> TRYIPDEADFLLGMATVNNCVSYRNPAEGTWYIQSLCQSLRERCPRGDDILTILTEVNY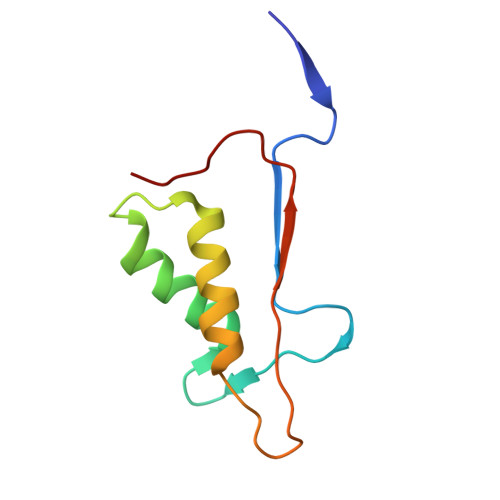EVSNKDDKKNMGKQMPQPTFTLRKKLVFP> MESKVVVPAQGKKITLQNGKLNVPENPIIPYIEGDGIGVDVTPAMLKVVDAAVEKAYKGERKISWMEIYTGEKSTQVYGQDVWLPAETLDLIREYRVAIKGPLTTPVGGGIRSLNVALRQELDLYICLRPVRYYQGTPSPVKHPELTDMVIFRENSEDIYAGIEWKADSADAEKVIKFLREEMGVKKIRFPEHC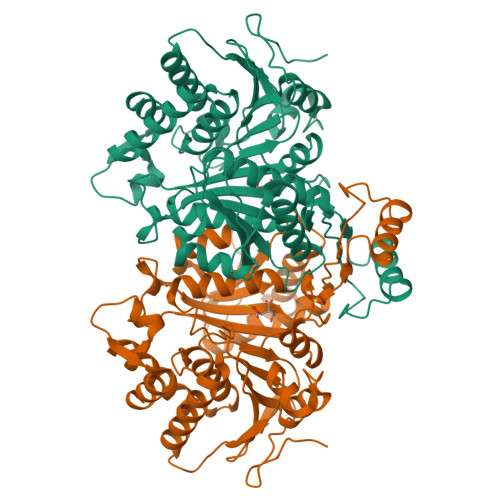GIGIKPCSEEGTKRLVRAAIEYAIANDRDSVTLVHKGNIMKFTEGAFKDWGYQLAREEFGGELIDGGPWLKVKNPNTGKEIVIKDVIADAFLQQILLRPAEYDVIACMNLNGDYISDALAAQVGGIGIAPGANIGDECALFEATHGTAPAYAGQDKVNPGSIILSAEMMLRHMGWTEAADLIVKGMEGAINAKTVTYDFERLMDGAKLLKCSEFGDAIIENM>[3x]PPGPPGPPGIPGEKGPAGE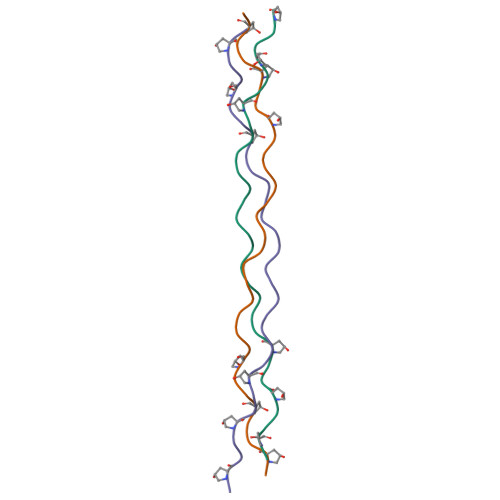RGPPGPPGPPG> MTDQNLPVTVAGLGPMGSALAA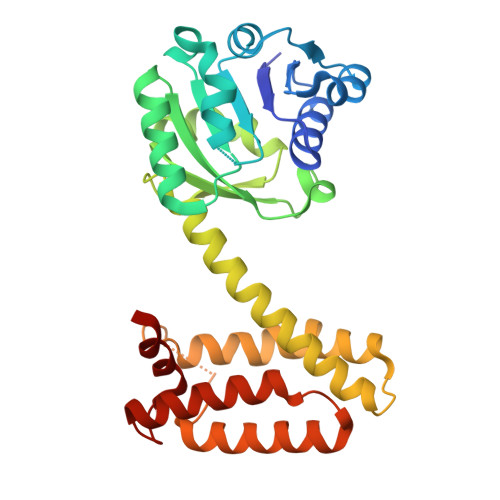ALLDRGHDVTVWNRSPGKAAPLVAKGARQADDIVDAVSASRLLVVCLADYDALYSALGPAREALRGRVVVNLNSGTPKEANEALRWAERHGTGYLDGAIMVPPAMVGHPGSVFLYSGSAEVFEEYKETLAGLGDPVHLGTEAGLAVLYNTALLSMMYSSMNGFLHAAALVGSAGVPAAEFTKLAVDWFLPAVIGQIIKAQAPTIDEGVYPGDAGSLEMNVTTLKHIIGTSQEQGVDTEIPVRNKELLDRAVAAGFGESSYYSVIELWR(3S,4S,5R)-3-(4-amino-3-bromo-5-fluorobenzyl)-5-{[3-(1,1-difluoroethyl)benzyl]amino}tetrahydro-2H-thiopyran-4-ol 1,1-dioxide | C21 H24 Br F3 N2 O3 S | 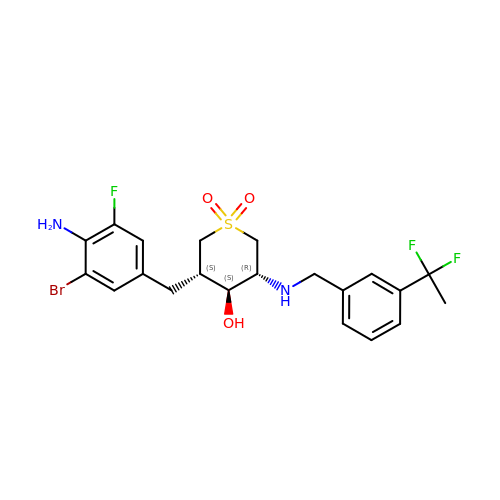QBRKIXCNLLQOPH-WNYOCNMUSA-N(5R)-3-(3,4-dichlorophenyl)-5-(4-hydroxyphenyl)-1,5-dimethyl-2-thioxoimidazolidin-4-one | C17 H14 Cl2 N2 O2 S | 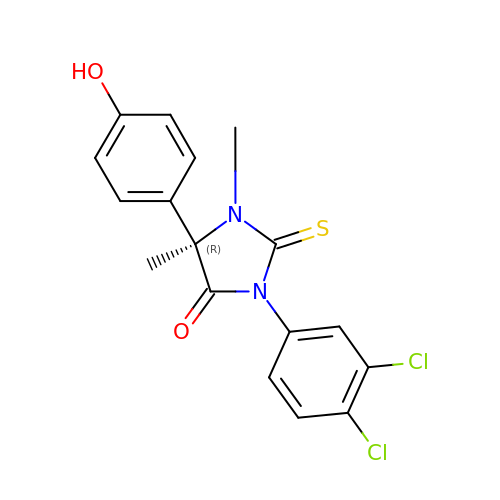YPONBLYNQFHCLA-QGZVFWFLSA-N> VGA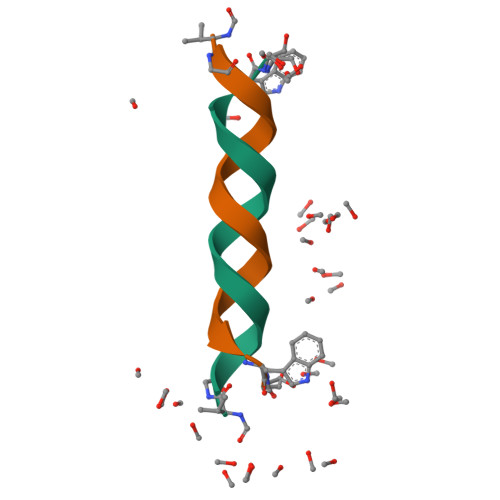LAVVVWLYLWLWX;> VGALAVVVWLWLWLWX>MDAQSAAKCLTAVRRHSPLVHSITNNVVTNFTANGLLALGASPVMAYAKEEVADMAKIAGALVLNIGTLSKESVEAMIIAGKSANEHGVPVILDPVGAGATPFRTESARDIIREVRLAAIRGNAAEIAHTVGVTD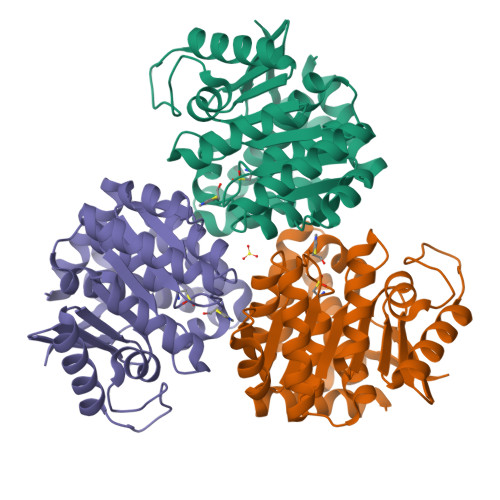WLIKGVDAGEGGGDIIRLAQQAAQKLNTVIAITGEVDVIADTSHVYTLHNGHKLLTKVTGAGCLLTSVVGAFCAVEENPLFAAIAAISSYGVAAQLAAQQTADKGPGSFQIELLNKLSTVTEQDVQEWATIERVTVS[2x]> SDPITGGHYENHNGYFVYIDASGKQVTGLQNIDGNLQYFDDNGYQVKGSFRDVNGKHIYFDSVTGKASSNVDIVNGKAQGYDAQGNQLKKSYVADSSGQTYYFDGNGQPLIGLQTIDGNLQYFNQQGVQIKGGFQDVNNKRIYFAPNTGNAVANTEIINGKLQGRDANGNQVKNAFSKDVAGNTFYFDANGVMLTGLQTISGKTYYLDEQGHLRKNYAGTFNNQFMYFDADTGAGKTAIEYQFDQGLVSQSNENTPHNAAKSYDKSSFENVDGYLTADTWYRPTDILKNGDTWTASTETDMRPLLMTWWPDKQTQANYLNFMSSKGLGITTTYTAATSQKTLNDAAFVIQTAIEQQISLKKSTEWLRDAIDSFVKTQANWNKQTEDEAFDGLQWLQGGFLAYQDDSHRTPNTDSGNNRKLGRQPINIDGSKDTTDGKGSEFLLANDIDNSNPIVQAEQLNWLHYLMNFGSITGNNDNANFDGIRVDAVDNVDADLLKIAGDYFKALYGTDKSDANANKHLSILEDWNGKDPQYVNQQGNAQLTMDYTVTSQFGNSLTHGANNRSNMWYFLDTGYYLNGDLNKKIVDKNRPNSGTLVNRIANSGDTKVIPNYSFVRAHDYDAQDPIRKAMIDHGIIKNMQDTFTFDQLAQGMEFYYKDQENPSGFKKYNDYNLPSAYAMLLTNKDTVPRVYYGDMYLEGGQYMEKGTIYNPVISALLKARIKYVSGGQTMATDSSGKDLKDGETDLLTSVRFGKGIMTSDQTTTQDNSQDYKNQGIGVIVGNNPDLKLNNDKTITLHMGKAHKNQLYRALVLSNDSGIDVYDSDDKAPTLRTNDNGDLIFHKTNTFVKQDGTIINYEMKGSLNALISGYLGVWVPVGASDSQDARTVATESSSSNDGSVFHSNAALDSNVIYEGFSNFQAMPTSPEQSTNVVIATKANLFKELGITSFELAPQYRSSGDTNYGGMSFLDSFLNNGYAFTDRYDLGFNKADGNPNPTKYGTDQDLRNAIEALHKNGMQAIADWVPDQIYALPGKEVVTATRVDERGNQLKDTDFVNLLYVANTKSSGVDYQAKYGGEFLDKLREEYPSLFKQNQVSTGQPIDASTKIKQWSAKYMNGTNILHRGAYYVLKDWATNQYFNIAKTNEVFLPLQLQNKDAQTGFISDASGVKYYSISGYQAKDTFIEDGNGNWYYFDKDGYMVRSQQGENPIRTVETSVNTRNGNYYFMPNGVELRKGFGTDNSGNVYYFDDQGKMVRDKYINDDANNFYHLNVDGTMSR;> KSYVADSSGQTYYFDGNGQPLIGLQTIDGNLQYFNQQGVQIKGGFQDVNNKRIYFAPNTGNAVANTEIINGKLQGRDANGNQVKNAFSKDVAGNTFYFDANGVMLTGLQTISGKTYYLDEQGHLRKNYAGTFNNQFMYFDADTGAGKTAIEYQFDQGLVSQSNENTPHNAAKSYDKSSFENVDGYLTADTWYRPTDILKNGDTWTASTETDMRPLLMTWWPDKQTQANYLNFMSSKGLGITTTYTAATSQKTLNDAAFVIQTAIEQQISLKKSTEWLRDAIDSFVKTQANWNKQTEDEAFDGLQWLQGGFLAYQDDSHRTPNTDSGNNRKLGRQPINIDGSKDTTDGKGSEFLLANDIDNSNPIVQAEQLNWLHYLMNFGSITGNNDNANFDGIRVDAVDNVDADLLKIAGDYFKALYGTDKSDANANKHLSILEDWNGKDPQYVNQQGNAQLTMDYTVTSQFGNSLTHGANNRSNMWYFLDTGYYLNGDLNKKIVDKNRPNSGTLVNRIANSGDTKVIPNYSFVRAHDYDAQDPIRKAMIDHGIIKNMQDTFTFDQLAQGMEFYYKDQENPSGFKKYNDYNLPSAYAMLLTNKDTVPRVYYGDMYLEGGQYMEKGTIYNPVISALLKARIKYVSGGQTMATDSSGKDLKDGETDLLTSVRFGKGIMTSDQTTTQDNSQDYKNQGIGVIVGNNPDLKLNNDKTITLHMGKAHKNQLYRALVLSNDSGIDVYDSDDKAPTLRTNDNGDLIFHKTNTFVKQDGTIINYEMKGSLNALISGYLGVWVPVGASDSQDARTVATESSSSNDGSVFHSNAALDSNVIYEGFSNFQAMPT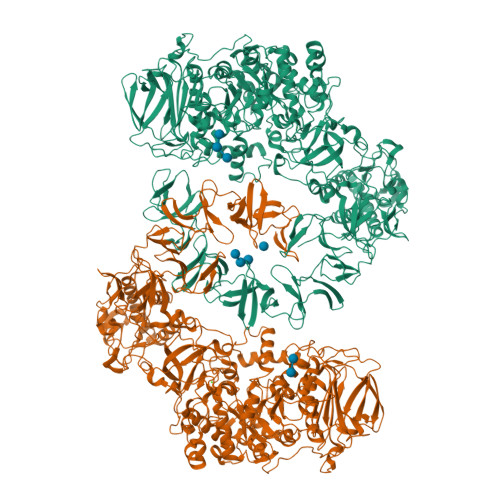SPEQSTNVVIATKANLFKELGITSFELAPQYRSSGDTNYGGMSFLDSFLNNGYAFTDRYDLGFNKADGNPNPTKYGTDQDLRNAIEALHKNGMQAIADWVPDQIYALPGKEVVTATRVDERGNQLKDTDFVNLLYVANTKSSGVDYQAKYGGEFLDKLREEYPSLFKQNQVSTGQPIDASTKIKQWSAKYMNGTNILHRGAYYVLKDWATNQYFNIAKTNEVFLPLQLQNKDAQTGFISDASGVKYYSISGYQAKDTFIEDGNGNWYYFDKDGYMVRSQQGENPIRTVETSVNTRNGNYYFMPNGVELRKGFGTDNSGNVYYFDDQGKMVRDKYINDDANNFYHLNVDGTMS>DYKDDDDKLDRADILYNIRQTSRPDVIPTQRDRPVAVSVSLKFINILEVNEITNEVDVVFWQQTTWSDRTLAWNSSHSPDQVSVPISSLWVPDLAAYNAISKPEVLTPQLARVVSDGEVLYMPSIRQRFSCDVSGVDTESGATCRIKIGSWTHHSREISVDPTTENSDDSEYFSQYSRFEILDVTQKKNSVTYSCCPEAYEDVEVSLNFRKKGRSEI[10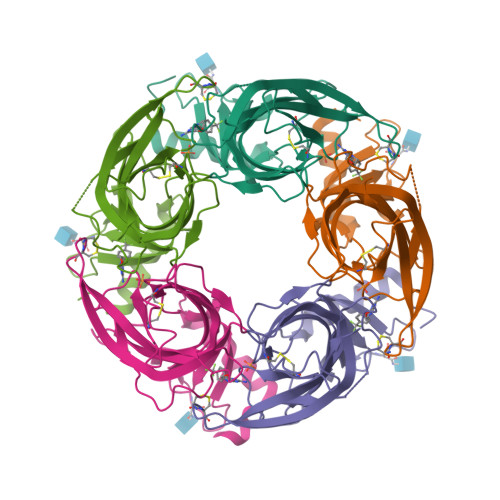x]> PPPPAQTFLFQGQPVVNRPLSLKDQQTFARSVGLKWRKVGRSLQRGCRALRDPALDSLAYEYEREGLYEQAFQLLRRFVQAEGRRATLQRLVEALEENELTSLAEDLLGLTDP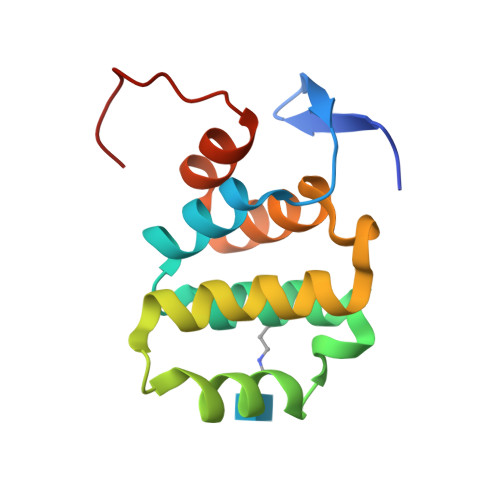NGGLA>GPAMATNGEIFNTYGHN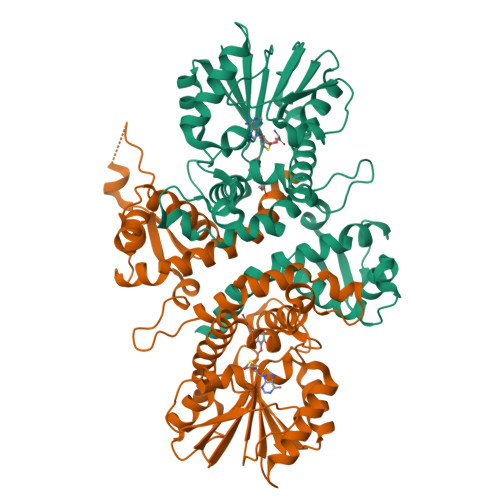HQSATVTKITASNESSNGVCYLSETANLGKLICIPMALRAAMELNVFQLISKFGTDAKVSASEIASKMPNAKNNPEAAMYLDRILRLLGASSILSVSTTAASINRGGDDVVVHEKLYGLTNSSCCLVPRQEDGVSLVEELLFTSDKVVVDSFFKLKCVVEEKDSVPFEVAHGAKIFEYAATEPRMNQVFNDGMAVFSIVVFEAVFRVYDGFLDMKELLDVGGGIGTSVSKIVAKYPLIRGVNFDLPHVISVAPQYPGVEHVAGDMFEEVPKGQNMLLKWVLHDWGDERCVKLLKNCWNSLPVGGKVLIIEFVLPNELGNNAESFNALIPDLLLMALNPGGKERTISEYDDLGKAAGFIKTIPIPISNGLHVIEFHK[2x]> MSTTQTPDLDAIVIGAGFGGIYMLHKLRNDLGLSVRVFEKGGGVGGTWYWNKYPGAKSDTEGFVYRYSFDKELLREYDWTTRYLDQPDVLAYLEHVVERYDLARDIQLNTEVTDAIFDEETELWRVTTAGGETLTARFLVTALGLLSRSNIPDIPGRDSFAGRLVHTNAWPEDLDITGKRVGVIGTGSTGTQFIVAAAKMAEQLTVFQRTPQYCVPSGNGPMDPDEVARIKQNFDSIWDQVRSSTVAFGFEESTVEAMSVSESERQRVFQQAWDKGNGFRFMFGTFCDIATNPEANAAAAAFIRSKIAEIVKDPETARKLTPTDLYAKRPLCNEGYYETYNRDNVSLVSLKETPIEEIVPQGVRTSDGVVHELDVLVFATGFDAVDGNYRAMNLRGRDGRHINEHWTEGPTSYLGVTKAGFPNMFMILGPNGPFTNTPPSIEAQVEWISDLIDKATREGLTTVEPTADAEREWTETCAEIANMTLFPK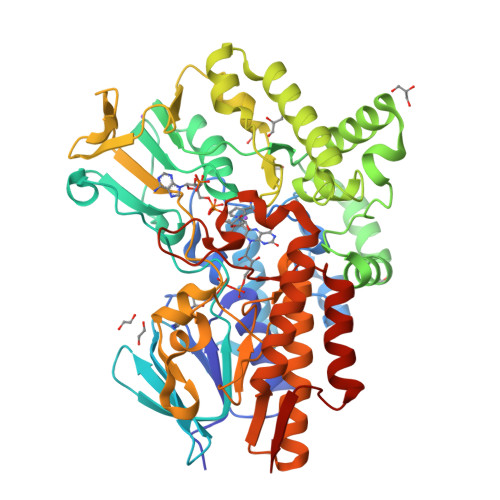ADSWIFGANIPGKRHAVMFYLGGLGNYRRQLADVADGGYRGFQLRGERAQAVA>SNAAAFKHVKSDIKIEKLNVTLNDAAKKQINNYTSQQVSNKKNDAWRDASATEIKSAMDSGTFIDNEKQKYQFLDLSKYQGIDKNRIKCMLVDRPTLLKHTDDFLKAAKDKHVNEVYLISHALLETGAVKSELANGVEIDGKKYYNFYGVGALDKDPIKTGAEYAKKHGWDTPEKAISGGADFIHKHFLSSTDQNTLYSMRWNPKNPGEHQYATDIKWAESNATIIADFYKNMKTEGKYFKYFVYKDDSKHLNK[2x]

Here, we present two crystal structures of GH73 enzymes from S. aureus, including glucosaminidase B (SagB) and the glucosaminidase part of major bifunctional autolysin (AtlA-gl). SagB crystallized with two and AtlA-gl with one molecule per asymmetric unit. In contrast to the crystal structure of AtlE and related N-acetylglucosaminidases, which were all observed in the closed form, these two proteins crystallized in the open form. Hence, for AtlA-gl and SagB to cleave a single glycan strand, both of their domains have to slide together into a closed conformation as observed in the AtlE structure.

SagB crystallized in the P6122 space group with two molecules per asymmetric unit. The structure of SagB is well-resolved based on electron density maps along the entire chain with the exception of the N36 to A41 region in both molecules, as indicated by the Ramachandran outliers and higher atomic B-values, as well as a few other side chains. The crystal structure also contains eight PEG molecules (PG4), two chloride ions and one sodium ion. The two molecules superimpose with a root-mean-square-deviation (RMSD) of 0.46 Å over all Cα atoms. The catalytic residue E121 is positioned at the C-terminus of helix α10. The R-domain comprises residues from A1 to D71 and S187 to K250, whereas the L-domain comprises residues from L72 to S186. The failure of molecular replacement was the first indication that the SagB structure must differ from the AtlE structure in spite of their high sequence similarity. Moreover, the angle of rotation of the SagB structure superimposed on the AtlE R-domain with the SagB structure superimposed onto the AtlE L-domain is 31° with a 3.5 Å screw translational component. Thus, the packing of the R-domains and L-domains in the SagB structure differs from their packing in the AtlE structure. The equivalent helix in the AtlE structure is distorted after the fourth turn with the aromatic residue Y201 slightly exposed. The α15 helix in SagB is almost a whole turn shorter and shares the same minor widening in the last turn of the helix at position F185.>APVKYGELIVLGYNGSLPNGDRGRRKSRFALFKRPKANGVKPSTVHIACTPQAAKAISNKDQHSISYTLSRAQTVVVEYTHDSNTDMFQIGRSTESPIDFVVTDTVPGSQSNSDTQSVQSTISRFACRIICERNPPFTARIYAAGFDSSKNIFLGEKAAKWKTSDGQMDGLTTNGVLVMHPRNGFTEDSKPGIWREISVCGNVFSLRETRSAQQRGKMVEIETNQLQDGSLIDLCGATLLWRTAEGLSHTP[2x];>[2x]AYEDSETQPFD

Pellino proteins are a small family of RING E3 ubiquitin ligases mainly involved in signaling events downstream of the Toll and interleukin-1 (IL-1) receptors (TIRs), which are key initiators of innate immune and inflammatory responses. All four members of the Pellino E3 ligase family contain atypic FHA domains at their N-terminus with conserved key amino acids known to be important for phospho-Threonine binding by canonical FHA domains. However, in contrast to the canonical FHA domain present in RNF8, Pellino FHA domains contain two substantial sequence inserts that extend from the FHA core and coalesce to form a wing-like subdomain. RNF8 itself is recruited to sites of DSBs by the adaptor protein MDC1, which in human cells, contains four conserved Thr-Gln-X-Phe motifs (TQXF motifs, where X stands for any amino acid).

Initial maps phased with just the molecular replacement model showed clear residual density for the MDC1-pT765 phosphopeptide and enabled a near-complete model of the complex to be built and refined at 2.7 Å resolution. The N-terminal fragment of PELI1 consists of 16 β-strands forming four distinct β-sheets, and a single α-helix. It features a central FHA core (residues 13–48, 97–156, and 183–257) comprising two β-sheets (β1-β2, β6-8, and β12-16) that form a β-sandwich. The FHA core is split by a bipartite “wing” appendage consisting of residues 45–96 (Wing I) and 157–182 (Wing II) consisting of the remaining two β-sheets (β3-5, β9, and β10-11) and an α-helix that separates β3-β4 and a large insertion between β3-β4. The MDC1-pT765 phosphopeptide binds in an extended conformation to a positively charged pocket within the PELI1-FHA domain, formed by loops separating β6-β7, β11-β12, and β14-β15. In total, the pT765 phosphate group forms four hydrogen-bonding interactions with side- and main-chain atoms from Arg104, Ser135, and Arg136 located in the loop separating β6-β7 of the FHA β-sandwich. The phosphate contacts made by Ser135 and Arg136 are highly conserved throughout the FHA family, including in RNF8 (Ser60 and Arg61) and Chk2 (Ser140 and Lys141) DDR proteins. The PELI1 wing domain does not make any contacts with the MDC1-pThr-765 phosphopeptide but instead acts as a structural support for a large insertion between β12-β13. This generates a shallow, positively charged platform formed predominantly by Arg 222 and Cys 247.>GSHSEQLKHCNGILKELLSKKHAAYAWPFYKPVDASALGLHDYHDIIKHPMDLSTVKRKMENRDYRDAQEFAADV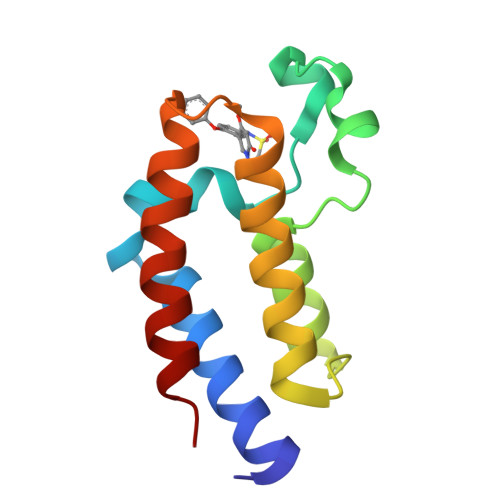RLMFSNCYKYNPPDHDVVAMARKLQDVFEFRYAKMP[2x]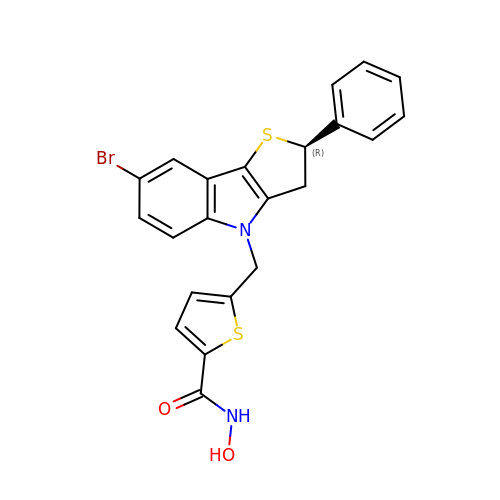5-[[(2R)-7-bromanyl-2-phenyl-2,3-dihydrothieno[3,2-b]indol-4-yl]methyl]-N-oxidanyl-thiophene-2-carboxamide | C22 H17 Br N2 O2 S2 | KZFHOXNMKKJROG-HXUWFJFHSA-N Kinesins are a large family of molecular motor proteins that utilize the energy from ATP hydrolysis to move along microtubules and transport various cellular cargoes. Zen4, MKLP1 (human homologue) and Pavarotti (Drosophila homologue) are kinesin-6 family proteins. They walk to and accumulate at the plus-end of interdigitated microtubules, playing a key role in formation of antiparallel central spindles during cytokinesis in animal cells. The kinesin-6 family proteins have two characteristic features: a long NL and a large insertion in the motor domain.

We crystallized the motor domain of Zen4 (1–441). The final structure was refined to 2.6 Å, with Rwork/Rfree=21%/24%. Interestingly, Zen4 is in the nucleotide-free, apo state. The structure reveals an ion, rather than a nucleotide, is bound by the P-loop (L4 loop). First, the ATPase catalytic site of Zen4 is in an open conformation, with the Switch I region (L9) moving away from the P-loop. Second, the N terminus of Switch II helix (α4) extends two helical turns and moves outward, consistent with enhanced microtubule binding in the apo state. Third, the nucleotide-binding pocket of Zen4 is occluded. In contrast, α6 of Zen4 is partially melted and ends at Phe419 (corresponding to Phe318 in kinesin-1), which is almost one helical turn shorter than the previous structure22. The NIS, starting from Glu421, flips backward, forms a five-residue β-strand and becomes disordered after Ile426. The backward flipping of NIS mainly occurs through backbone hydrogen-bond interactions with the N-terminal β1c strand, becoming a part of the N-terminal antiparallel appending β-sheet.

>[2x]GHMGSSGGMSSRKRGITPSRDQVRRKKLSIEETDSIEVVCRLCPYTGSTPSLIAIDEGSIQTVLPPAQFRRENAPQVEKVFRFGRVFSENDGQATVFERTSVDLILNLLKGQNSLLFTYGVTGSGKTYTMTGKPTETGTGLLPRTLDVIFNSINNRVEKCIFYPSALNTFEIRATLDAHLKRHQMAADRLSTSREITDRYCEAIKLSGYNDDMVCSVFVTYVEIYNNYCYDLLEDARNGVLTKREIRHDRQQQMYVDGAKDVEVSSSEEALEVFCLGEERRRVSSTLLNKDSSRSHSVFTIKLVMAPRAYETKSVYPTMDSSQIIVSQLCLVDLAGSERAKRTQNVGERLAEANSINQSLMTLRQCIEVLRRNQKSSSQNLEQVPYRQSKLTHLFKNYLEGNGKIRMVICVNPKPDDYDENMSALAFAEESQTIEVKKQVERMPSERIP> MSDVAIVKEGWLHKRGEYIKTWRPRYFLLKNDGTFIGYKERPQDVDQREAPLNNFSVAQCQLMKTERPRPNTFIIRCLQWTTVIERTFH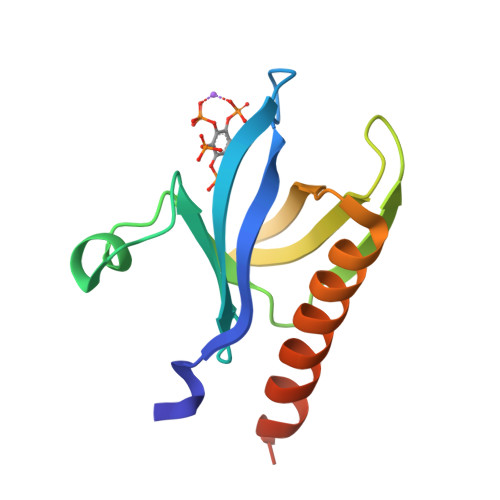VETPEEREEWTTAIQTVADGLKKQEEEEMDFRSG>ISLGELGLLPSTVLAIGYYENFVSTVCDALHSLPTIKLNGIEYKDFVFNIIIPNDLDADIKRRAQIYFKKMDIHEVKIDTNGRSFPLYLQIDEENSGDVAVLYDMPTTLGGIDKAIEMYMKKGHIGKTSQQQLLEERELRNFKTTLINLINNNSFTKTFVKVIEE[4x]

A recent groundbreaking study discovered the ancient origins of the cGAS-STING pathway in bacteria, which play a similar role in the immune system to combat bacteriophage infections. Binding of cGG to bacterial STING causes it to oligomerize into long filaments and activates the nicotinamide adenine dinucleotide (NAD)+ cleavage activity of its fused N-terminal Toll/interleukin-1 receptor (TIR) domain. Depletion of the electron carrier NAD+ eventually leads to bacterial growth arrest or cell death, restricting the replication of invading phages in infected bacteria, a strategy called “abortive infection. In this study, we demonstrated two distinct mechanisms underlying the regulation of bacterial STINGs and a structural basis for cAA recognition and oligomerization.

Epilithonimonas lactis STING (ElSTING) was identified to bind cAA with micromolar affinity. To reveal the molecular mechanism underlying cAA recognition by ElSTING, we determined the 2.57 Å and 2.55 Å crystal structures of ligand-free and cAA-bound form of ElSTING, respectively, which forms canonical V-shaped dimer conformations. Binding of cAA stabilizes the formation of the β-strand lid and further induces complete lid closure to seal the ligand-binding pocket of ElSTING. This results in formation of a more compact dimeric architecture than cGG-bound bacterial STINGs. Recognition of cAA by ElSTING is mainly through shape complementarity. In particular, the hydrophobic sidechain of Y165, F169, and L234, a lid residue P233 along with phosphate-backbone-interacting residues N168, T254, and T255 together constitute a more compact and limited ligand-binding pocket to clamp cAA inside. In contrast to the cGG binding mode, there is no room leaving for cation-π or π-π interactions between the sidechain of R230/F232 and the bound cAA. As a result, the bound cAA formed a self-stacked, triangle-shaped conformation in which the two adenine bases came close to each other by inward rotation of 26° and shortened the distance between the 6-NH2 group of the adenine bases to 3.3 Å in comparison with 5.4 − 6.7 Å of the U-type cAA bound in eukaryotic STINGs. The base recognition of cAA by ElSTING was mediated via indirect hydrogen bonding through water molecules: w1 and w2 bridges the side-chains of the D251 and N3 atoms of the adenine base, whereas w3 mediates the hydrogen bonding between the main-chain of N168 and the N7 atom of the adenine base. Binding of cAA induced lid closure of ElSTING, which further oligomerizes into spiral-shaped filaments via lateral dimer-dimer interactions with a rotation of 30° per dimer along the direction of filament extension.> GPASGEGKKVDIAGIYPPVTTPFTATAEVDYGKLEENLHKLGTFPFRGFVVQGSNGEFPFLTSSERLEVVSRVRQAMPKNRLLLAGSGCESTQATVEMTVSMAQVGADAAMVVTPCYYRGRMSSAALIHHYTKVADLSPIPVVLYSVPANTGLDLPVDAVVTLSQHPNIVGM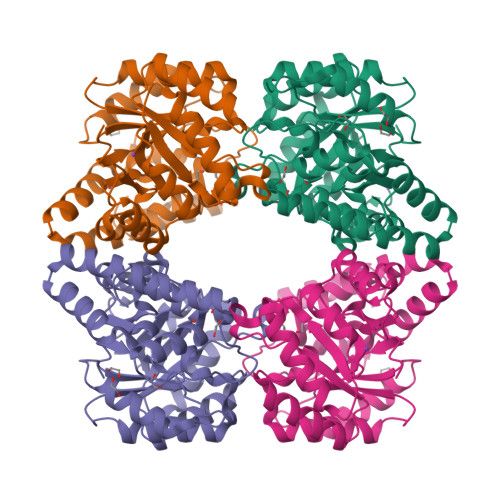KDSGGDVTRIGLIVHKTRKQDFQVLAGSAGFLMASYALGAVGGVCALANVLGAQVCQLERLCCTGQWEDAQKLQHRLIEPNAAVTRRFGIPGLKKIMDWFGYYGGPCRAPLQELSPAEEEALRMDFTSNGWL> MDPYCPFDALD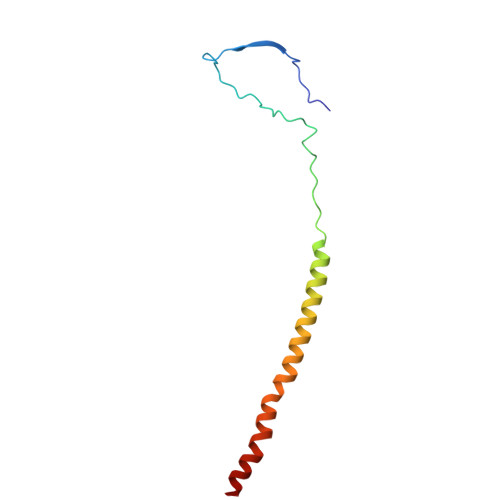VWEHRRFIVADSRNFITPEFPRDFWMSPVFNLPRETAAEQVVVLQAQRTAAAAALENAAMQAAELPVDIERRLRPIERNVHEI>MDDANKIRREEVLVSMCDQRARMLQDQFSVSVNHVHALAILVSTFHYHKNPSAIDQETFAEYTARTAFERPLLSGVAYAEKVVNFEREMFERQHNWVIKTMDRGEPSPVRDEYAPVIFSQDSVSYLESLDMMSGEEDRENILRARETGKAVLTSPFRLLETHHLGVVLTFPVYKSSLPENPTVEERIAATAGYLGGAFDV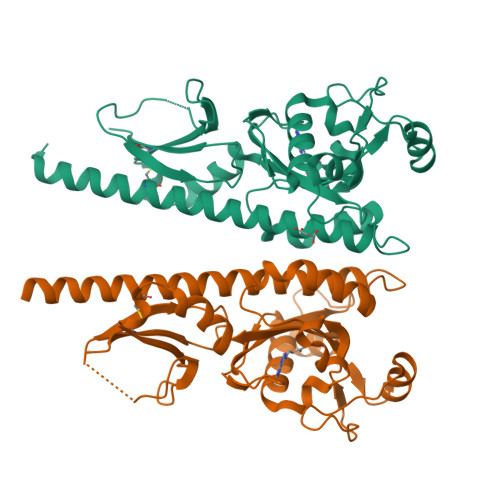ESLVENLLGQLAGNQAIVVHVYDITNASDPLVMYGNQDEEADRSLSHESKLDFGDPFRKHKMICRYHQKA[2x]> GLPTMNTPGSNQFLTSDDFQSPSAMPQFDVTPEMHIPGEVRNLMEIAEVD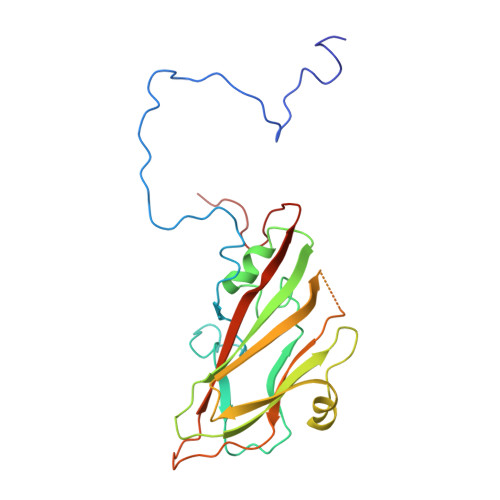SVMPINNDSAAKVSSMEAYRVELSTNTNAGTQVFGFQLNPGAESVMNRTLMGEILNYYAHWSGSIKITFVFCGSAMTTGKFLLSYAPPGAGAPKTRKDAMLGTHVVWDVGLQSSCVLCIPWISQTHYRFVEKDPYTNAGFVTCWYQTSVVSPASNQPKCYMMCMVSACNDFSVRMLRDTKFIEQTSFYQ(5S,9R,10R,12S)-12-[3-(AMINOMETHYL)PHENYL]-5-BENZYL-10-HYDROXY-9-ISOPROPYL-3-OXO-1-PHENYL-2-OXA-7-THIA-4,8-DIAZA-10-PHOSPHATRIDECAN-13-OIC 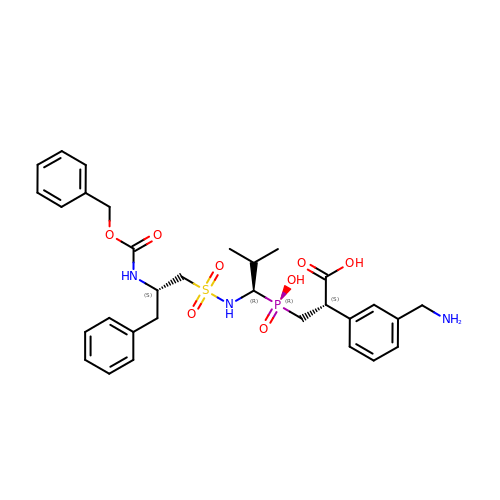ACID 7,7,10-TRIOXIDE | C31 H40 N3 O8 P S | FGYZBAFIDVPVGG-YTCPBCGMSA-N> DKATIPSESPFAAAEVADGAIVVDIAKMKYETPELHVKVGDTVTWINREAMPHNVHFVAGVLGEAALKGPMMKKEQAYSLTFTEAG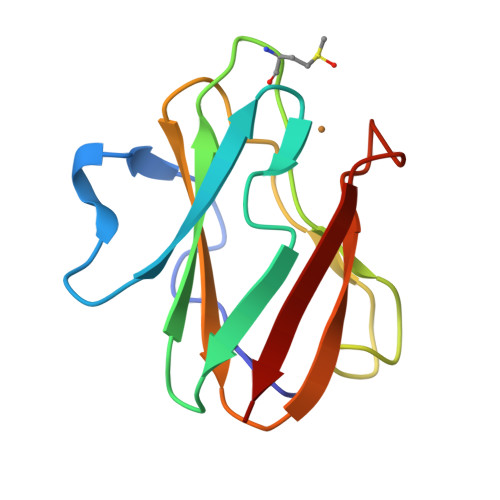TYDYHCTPHPFQRGKVVVE> MNHKVHHHHHHIEGRHMINNKFAVSTISDYTEKINNVKDEEVDDLIKNINKYNYDLFNGTAENQLPDYLNIHEGDVLGYIEIPSINIKLPIYYGTSVDILKKGVGVLEGTSLPVGGENTHSVLSAHTGLANQKLFTDIDKLKDGDVFYLHILKKDLAYKVNQIKVVHPDEIDELKISDDKDYVTLLTCYPYGINTERLLVRGERTDLSPSNGAGFS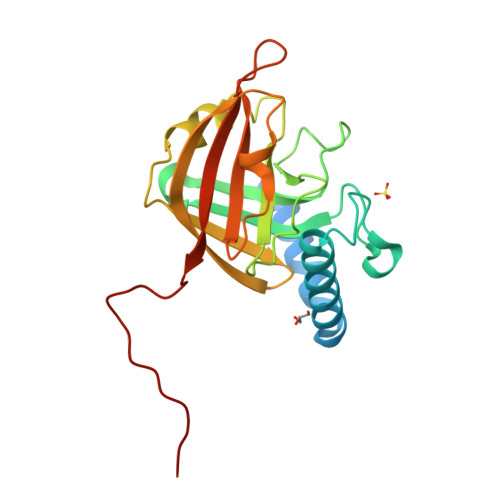LPST>[2x]MEGMRRPTPTVYVGRVPIG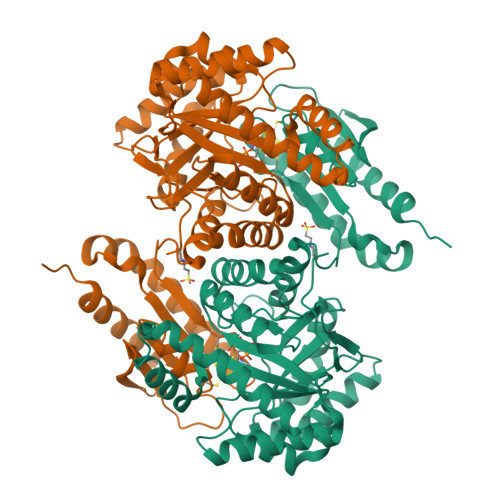GAHPIAVQSMTNTPTRDVEATTAQVLELHRAGSEIVRLTVNDEEAAKAVPEIKRRLLAEGVEVPLVGDFHFNGHLLLRKYPKMAEALDKFRINPGTLGRGRHKDEHFAEMIRIAMDLGKPVRIGANWGSLDPALLTELMDRNASRPEPKSAHEVVLEALVESAVRAYEAALEMGLGEDKLVLSAKVSKARDLVWVYRELARRTQAPLHLGLTEAGMGVKGIVASAAALAPLLLEGIGDTIRVSLTPSPKEPRTKEVEVAQEILQALGLRAFAPEVTSCPGCGRTTSTFFQELAEEVSRRLKERLPEWRARYPGVEELKVAVMGCVVNGPGESKHAHIGISLPGAGEEPKAPVYADGKLLTILKGEGIAEEFLRLVEDYVKTRFAPKA>GQQMETGDQRFGDLVFRQLAPNVWQHTSYLDMPGFGAVASNGLIVRDGGRVLVVDTAWTDDQTAQILNWIKQEINLPVALAVVTHAHQDKMGGMDALHAAGIATYANALSNQLAPQEGMVAAQHSLTFAANGWVEPATAPNFGPLKVFYPGPGHTSDNITVGIDGTDIAFGGCLIKD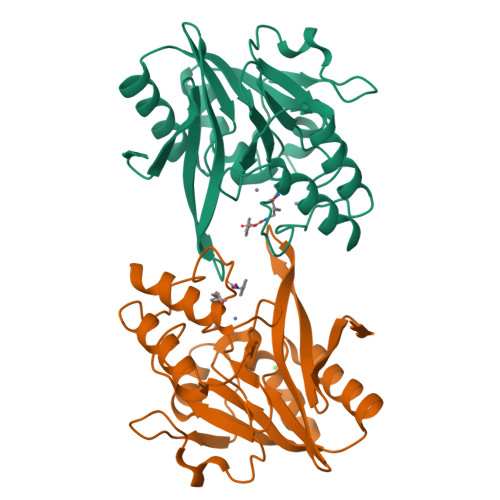SKAKSLGNLGDADTEHYAASARAFGAAFPKASMIVMSHSAPDSRAAITHTARMADKLR[2x]> EMAESVSRPQRPPVIWIGAQECTGCTESLLRATHPTVENLVLETISLEYHEVLSAAFGHQVEENKHNALEKYKGQYVLVVDGSIPLKDNGIYCMVAGEPIVDHIRRAAEGAAAIIAIGSCAAWGGVAAAGVNPTGAVGLQEVLPGKTIINIPGCPPNPHNFLATVAHIITYGKPPKLDAKNRPTFAYGRLIHEHCERRPHFDAGRFAKEFGDEGHREGWCLYHLGCKGPETYGNCSTLQFCDVGGVWPVAIGHPCYGCNEEGIGFHKGIHQLAHVENQTPRSEKPDVNIKEGGNISAGAVGLLGGVVGLVAGVSVMAVRELGRQ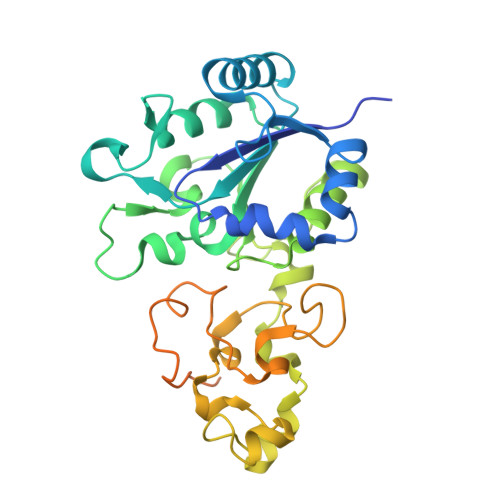QKKDNADSRGE> MGKVILVTGVSRGIGKSIVDVLFSLDKDTVVYGVARSEAPLKKLKEKYGDRFFYVVGDITEDSVLKQLVNAAVKGHGKIDSLVANAGVLEPVQNVNEIDVNAWKKLYDINFFSIVSLVGIALPELKKTNGNVVFVSSDACNMYFSSWGAYGSSKAALNHFAMTLANEERQVKAIAVAPGIVDTDMQVNIRENVGPSSMSAEQLKMFRGLKENNQLLDSSVPATVYAKLALHGIPDGVNGQY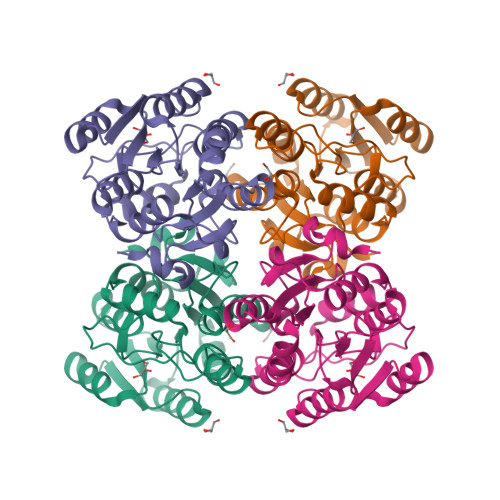LSYNDPALADFMP> GSALRELKVCLLGDTGVGKSSIMWRFVEDSFD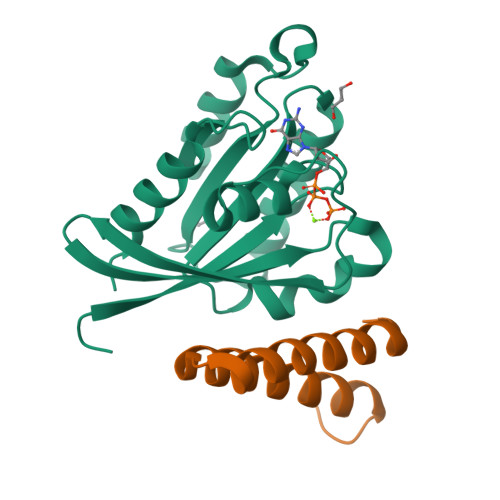PNINPTIGASFMTKTVQYQNELHKFLIWDTAGLERFRALAPMYYRGSAAAIIVYDITKEETFSTLKNWVRELRQHGPPSIVVAIAGNKCDLTDVREVMERDAKDYADSIHAIFVETSAKNAININELFIEISRRIPST;> GSPEAEEPIEEELLLQQIDNIKAYIFDAKQCGRLDEVEVLTENLRELKHTLAKQKGGTD>MNYPAEPFRIKSVETVSMIPRDERLKKMQEAGYNTFLLNSKDIYIDLLTDSGTNAMSDKQWAGMMMGDEAYAGSENFYHLERTVQELFGFKHIVPTHQGRGAENLLSQLAIKPGQYVAGNMYFTTTRYHQEKNGAVFVDIVRDEAHDAGLNIAFKGDIDLKKLQKLIDEKGAENIAYICLAVTVNLAGGQPVSMANMRAVRELTAAHGIKVFYDATRCVENAYFIKEQEQGFENKSIAEIVHEMFSYADGCTMSGKKDCLVNIGGFLCMNDDEMFSSAKELVVVYEGMPSYGGLAGRDMEAMAIGLREAMQYEYIEHRVKQVRYLGDKLKAAGVPIVEPVGGHAVFLDARRFCEHLTQDEFPAQSLAASIYVETGVRSMERGIISAGRNNVTGEHHRPKLETVRLTIPRRVYTYAHMDVVAD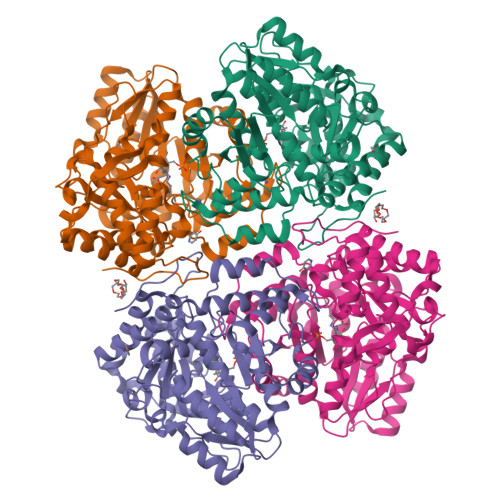GIIKLYQHKEDIRGLKFIYEPKQLRFFTARFDYI[2x]>SNAMEIKSILIANRGEIALRALRTIKEMGKKAICVYSEADKDALYLKYADASICIGKARSSESYLNIPAIIAAAEIAEADAIFPGYGFLSENQNFVEICAKHNIKFIGPSVEAMNLMSDKSKAKQVMQRAGVPVIPGSDGALAGAEAAKKLAKEIGYPVILKAAAGGGGRGMRVVENEKDLEKAYWSAESEAMTAFGDGTMYMEKYIQNPRHIEVQVIGDSFGNVIHVGERDCSMQRRHQKLIEESPAILLDEKTRTRLHETAIKAAKAIGYEGAGTFEFLVDKNLDFYFIEMNTRLQVEHCVSEMVSGIDIIEQMIKVAEGYALPSQESIKLNGHSIECRITAEDSKTFLPSPGKITKYIPPAGRNVRMESHCYQDYSVPAYYDSMIGKLVVWAEDRNKAIAKMKVALDELLISGIKTTKD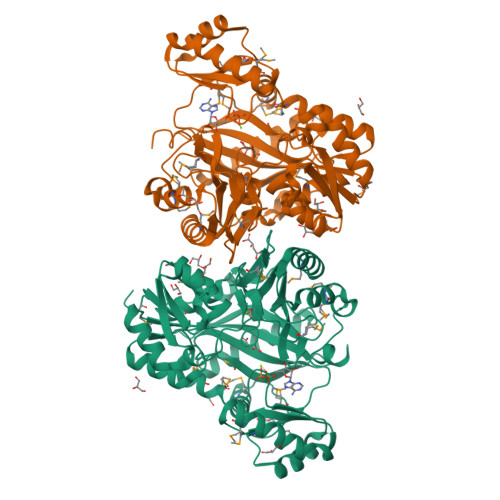FHLSMMENPDFINNNYDTNYLARH[2x]> GEKTYVKRLVKILLLGAGESGKSTFLKQMRIIHGQDFDQRAREEFRPTIYSNVIKGMRVLVDAREKLHIPWGDNKNQLHGDKLMAFDTRAPMAAQGMVETRVFLQYLPAIRALWEDSGIQNAYDRRREFQLGESVKYFLDNLDKLGVPDYIPSQQDILLARRPTKGIHEYDFEIKNVPFKMVDVGGLRSERKRWFECFDSVT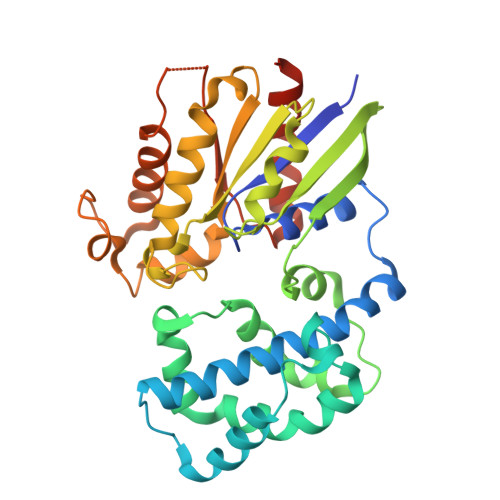SILFLVSSSEFDQVLMEDRQTNRLTESLNIFETIVNNRVFSNVSIILFLNKTDLLEEKVQVVSIKDYFLEFEGDPHCLRDVQKFLVECFRGKRRDQQQRPLYHHFTTAINTENIRLVFRDVKDTILHDNLKQLMLQ> MASQRLFVLDNERYDSFITQLEAP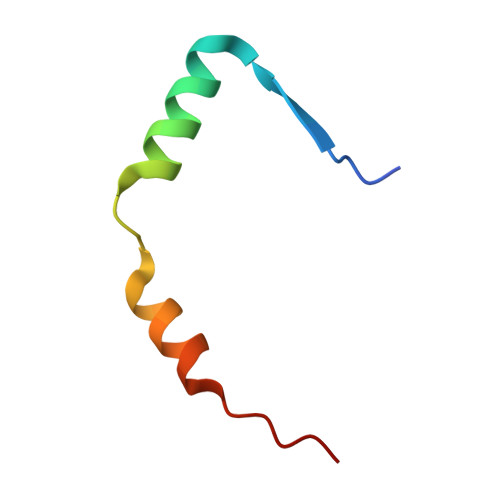VQNAEGRERLMAVKPEWK>[4x]GHHHHHHHHIEGRSLDPTVHWLFTTCGASGPHGPTQAQCNNAYQNSNLSVEVGSEGPLKGIQIWKVPATDTYSISGYGAAGGKGGKNTMMRSHGVSVLGIFNLEKDDMLYILVGQQGEDACPSTN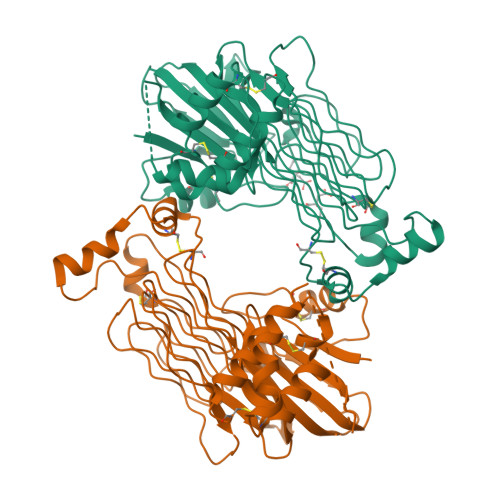QLIQKVCIGENNVIEEEIRVNRSVHEWAGGGGGGGGATYVFKMKDGVPVPLIIAAGGGGRAYGAKTDTFHPERLENNSSVLGLNGNSGAAGGGGGWNDNTSLLWAGKSLQEGATGGHSCPQAMKKWGWETRGGFGGGGGGCSSGGGGGGYIGGNAASNNDPEMDGEDGVSFISPLGILYTPALKVMEGHGEVNIKHYLNCSHCEVDECHMDPESHKVICFCDHGTVLAEDGVSCIVSPTPEPHGGSGGSGGSGGSGGAEIVPRDLRMKDKFLKHLTGPLYFSPKCSKHFHRLYHNTRDCTIPAYYKRCARLLTRLAVSPVCMEDKQ>[2x]DWVIPPISCPENEKGEFPKNLVQIKSNRDKETKVFYSITGQGAD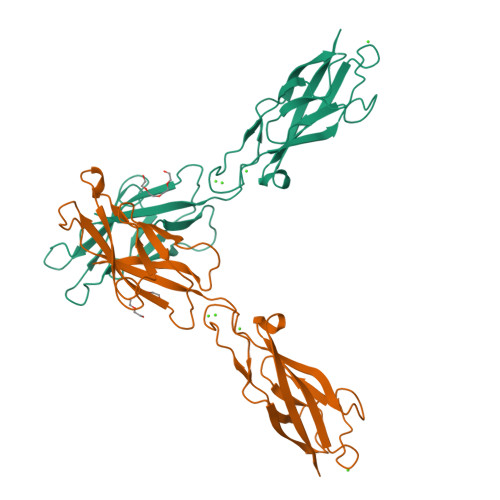KPPVGVFIIERETGWLKVTQPLDREAIAKYILYSHAVSSNGEAVEDPMEIVITVTDQNDNRPEFTQEVFEGSVAEGAVPGTSVMKVSATDADDDVNTYNAAIAYTIVSQDPELPHKNMFTVNRDTGVISVDTSGLDRESYPTYTLVVQAADLQGEGLSTTAKAVITVKD> DDVSISPEQSFYEIMLIRPKTIDDINYVVDQVLEESNPVILDLSFLEKESPANFKLAGEKIKQMRSNYGAEALLLSRCNDKNLIIIAPKGVSLVRK

Here, we combine structural, cellular, and evolutionary analyses to demonstrate that SepF is the FtsZ anchor in the human-associated archaeon Methanobrevibacter smithii. M. smithii SepF binds to membranes and to FtsZ, inducing filament bundling. High-resolution crystal structures of archaeal SepF alone and in complex with the FtsZ C-terminal domain (FtsZCTD) reveal that SepF forms a dimer with a homodimerization interface driving a binding mode that is different from that previously reported in bacteria.

We determined the crystal structure of MsSepFcore, at 1.4 Å resolution. The protein is a dimer in solution, with each protomer consisting of a 5-stranded β-sheet flanked by 2 α-helices. In addition, a helical turn insertion (η1), between strand β2 and helix α2, is conserved in archaeal sequences but is absent in bacterial homologs. Despite their quite similar monomeric structure, the dimeric arrangement of archaeal SepF differs from that observed for the functional dimer in CgSepF, where the dimer interface is formed by a 4 α-helical bundle. Interestingly, the functional dimer (as defined by its complex with FtsZ) strikingly differs between MsSepF, where it is formed via a β-β interface, and CgSepF, where it is formed via an α-α interface. Importantly, a bacterial-like α-α interface is not possible in archaeal SepF because a crucial glycine residue (Gly114 in CgSepF) buried at the center of the bacterial interface is substituted by charged residues with longer side chains (Lys, Glu, Asp) in archaeal sequences, precluding such interaction to occur. However, the only other available bacterial SepF structure (CgSepF) revealed that a C-terminal helix α3 interacts with the β-sheet of SepF and would therefore preclude formation of a β-β interface. Remarkably, helix α3 is predicted to be conserved in most bacterial sequences including B. subtilis, but not in Archaea. In fact, we (and others) did not obtain conclusive experimental evidence that MsSepF polymerizes, and the three available archaeal SepF structures provide no hints about a possible mechanism.>[2x]GPGSMTVVEAKSRIAVVGGGGSGSVAAWLLARRHDVTLFEADEYLGGHAYSHPVETDQGTLHVDMGVQHFNEKLSPNLFRLLTDFGIGTYVAPSSVHVDFPGEQQSWNNLDFLGELREELHEEFDRFHQEMNQLPTSGDDSYKQMSIGEYLDKHGYSKSFKYKAMNPILSIYSGCHAPSL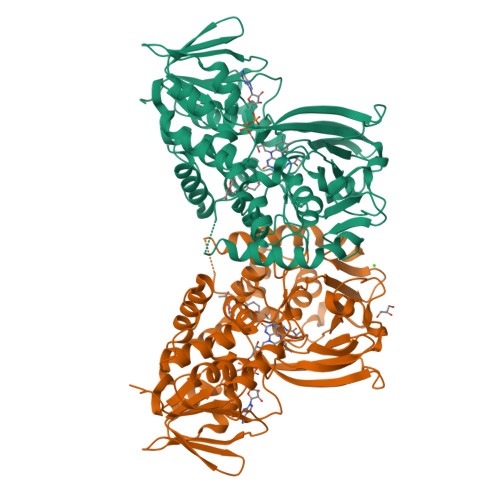DYNLMYVALSFSMNLLSFFSAGYWRKAQGGIHSYLARIESDLGERVRLNTPVEAVVPTQSGVTVLAGGQEHHFDQVVFATHADVTLRLLRTSDQQYRDLLGDFAYVPVESVLHQDESWLSPAGGGAYCQFRMPEGFELARAEEQMGSLTRNCNVLHPYRKVSSPILITFDPQEDVDPERVIVRREWKLPQLRPVDVRRKKRLHEIQGLNGLWFCGTDTSVTGHEGAIVSGMVIADRLGVPHPFPDDAPAAAQFRGIKEFMGV>[3x]MKRREVLQTAASALVGALSVSTFSSYAAKNTGLALKSVDATAIPKGDVPILTPENVYAMPPQFWQNFQGKLWIGRAGSDARQPGNQIPVFLRDANGNLAQITQPITLNKGNFDQFVKDNAALIANPSHAMALEDSNGQTVFNIPDVS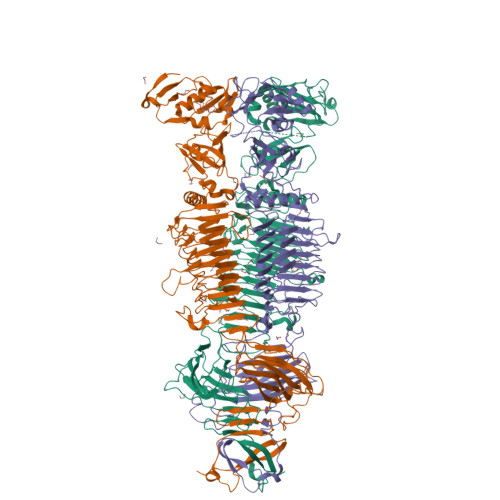QPGQAAFSQRLAQPAGYQLIGEIPSVDDLRKTRPLFEGAKIKLKSWHPGLEVGGGEFVGSFQPAQDDQGVIFSGDGFHWRRVVDDYNRLSLFDFGAIADGKTDSAPAIKAMYQWSQQSDQPICVQFPAGTFFVTGCDFGEEQRRFFRISGAMVNFGYFPATTIVSDGQSPFVFEVSARWVEISNLIFNGNTDTKPNRQGLLRNTCPGGQFFRGACLRFNNVGGTALSLLDTLDCKIDQWYASACTGDVIQAGWSGQKKGNWDHSTAIELSNFNAQHCKGGKVLNLPRCSQSLIHNGWIEHCDNPGDISNGQWIIDALSLEDCKNPLIAWHSRLNTRQTNLQSGSWIDNSEQGDRWLSAWEMGSTRVESYGVAIDGSLKYNYLTSRWLLENNTSQPVWYELANLYSPTVGDSWEIEVFGQSQFNNGTDSEPLMNLIDGRNTGGRAVIHVQRKKDHAEASWSAEGSSPVLDVRYVAKTDTDTQVFIRLAGWTPSAAIMIKSTAKDRFVTGRCARVDAKMAKATPDSGSHAAPQRFSLHNGKAGVGANEQGDLLLASRALSADNVDTRKPEGFVSVVINGKTVALPYFAIKA>[2x]MA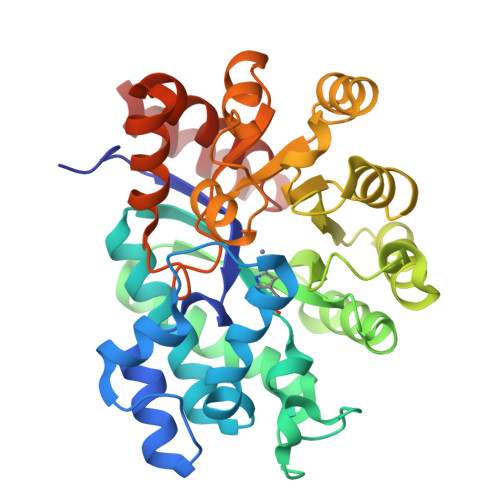QTPAFNKPKVELHVHLDGAIKPETILYFGKKRGIALPADTVEELRNIIGMDKPLSLPGFLAKFDYYMPVIAGCREAIKRIAYEFVEMKAKEGVVYVEVRYSPHLLANSKVDPMPWNQTEGDVTPDDVVDLVNQGLQEGEQAFGIKVRSILCCMRHQPSWSLEVLELCKKYNQKTVVAMDLAGDETIEGSSLFPGHVEAYEGAVKNGIHRTVHAGQVGSPEVVREAVDILKTERVGHGEHTIEDEALYNRLLKENMHFEVCPWSSYLTGAWDPKTTHAVVRFKNDKANYSLNTDDPLIFKSTLDTDYQMTKKDMGFTEEEFKRLNINAAKSSFLPEEEKKELLERLYREYQ>[2x]MVVKFMDVYQRSYCHPIETLVDIFQEYPD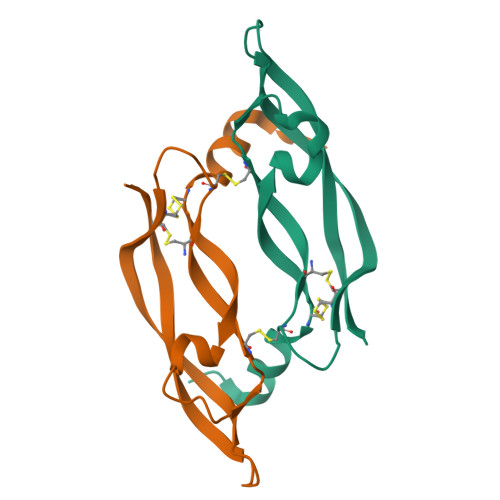EIEYIFKPSCVPLMRCGGCANDEGLECVPTEESNITMQIMRIKPHQGQHIGEMSFLQHNKCEARPKK>[2x]G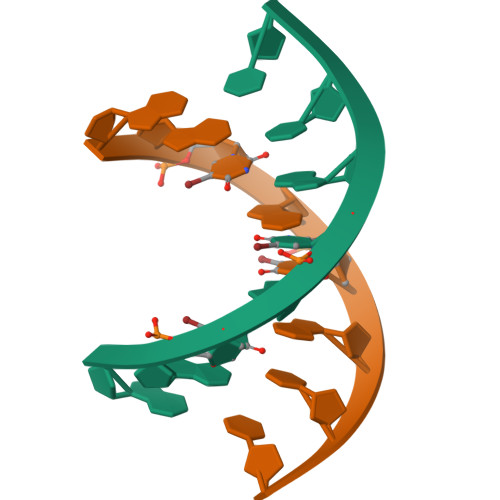GUAUACC> MEYGHHARPDSKRPLDEGSPAAAGLTSKKANEALTRNRELTTVLVKNLPKSYNQNKVYKYFKHCGPIIHVDVADSLKKNFRFARIEFARYDGALAAITKTHKVVGQNEIIVSHLTECTLWMTNFPPSYTQRNIRDLLQDINVVALSIRLPSLRFNTSRRFAYIDVTSKEDARYCVEKLNGLKIEGYTLVTKVSNPLEKSKRTDSATLEGREIMIRNLSTELLDENLLRESFEGFGSIEKINIPAGQKEHSFNNCCAFMVFENKDSAERALQMNRSLLGNREISVSLADKKPFLERNEVKRLLASRNSKELETLICLFPLSDKVSPSLICQFLQEEIHINEKDIRKILLVSDFNGAIIIFRDSKFAAKMLMILNGSQFQGKVIRSGTINDMKRYYNNQQNHSMKHVKPSCINMMEKGPNLQVKKKIPDKQEQMSNDDFRKMFLGELEHHHHHH;> MGSMLFFSFFKTLVDQEVVVELKNDIEIKGTLQSVDQFLNLKLDNISCTDEKKYPHLGSVRNIFIRGSTVRYVYLNKNMVDTNLLQDATRREVMTERK;> MGSMETPLDLLKLNLDERVYIKLRGARTLVGTLQAFDSHCNIVLSDAVETIYQLNNEELSESERRCEMVFIRGDTVTLISTPSEDDDGAVEI;> MGSMLPLYLLTNAKGQQMQIELKNGEIIQGILTNVDNWMNLTLSNVTEYSEESAINSEDNAESSKAVKLNEIYIRGTFIKFIKLQDNIIDKVKQQI;> MGSMSLPEILPLEVIDKTINQKVLIVLQSNREFEGTLVGFDDFVNVILEDAVEWLIDPEDESRNEKVMQHHGRMLLSGNNIAILVPGGKKTPTEAL;> GSMSGKASTEGSVTTEFLSDIIGKTVNVKLASGLLYSGRLESIDGFMNVALSSATEHYESNNNKLLNKFNSDVFLRGTQVMYISEQKI;> MGSMHQQHSKSENKPQQQRKKFEGPKREAILDLAKYKDSKIRVKLMGGKLVIGVLKGYDQLMNLVLDDTVEYMSNPDDENNTELISKNARKLGLTVIRGTILVSLSSAEGSDVLYMQK;> GSMSATLKDYLNKRVVIIKVDGECLIASLNGFDKNTNLFITNVFNRISKEFICKAQLLRGSEIALVGLIDAENDDSLAPIDEKKVPMLKDTKNKIENEHVIWEKVYESKTK

Thus, U6 recruitment into spliceosomes proceeds though a novel, and poorly understood, RNA remodeling mechanism involving large-scale conformational changes. The core region of the U6 snRNP retains the unique “interlocked rings” topology of Prp24 and U6 snRNA and is virtually identical to previously determined structures of U6/Prp24 binary complexes, with a comparative r.m.s.d of ~1.3 Å. There are protein–protein contacts in the U6 snRNP that were not visible in previous structures, including a 660 Å2 contact between RRM4 of Prp24 and Lsm2, and a contact between the conserved C-terminus (or “SNFFL box”) of Prp24 and Lsm5 and Lsm7. The architecture of the free U6 snRNP provides insights into how spliceosomal RNAs can be remodeled in the absence of an ATP-dependent helicase.

Inside the ring, RNA is bound in a shifted register relative to that observed previously. Instead of being bound in the Sm-like pocket of Lsm3, the terminal nucleotide occupies a new pocket comprised of residues in Lsm2, Lsm3 and Lsm8, and the penultimate nucleotide is bound in the previously identified Sm-like pocket of Lsm3.> GAPATVTEQGEDITSKKDRGVLKIVKRVGNGEETPLIGDKVYVHYKGKLSNGKKEDSSHDRNEPFVFSLGKGQVIKAWDIGVATLKKGEIAHLLIKPEYAYGSAGSLPKIPSNATLFFEIELLDFKGE

Here we used the FK506-binding protein 51 (FKBP51) as a model system to evaluate whether chemically engineered proteins can be trapped in pharmacologically relevant conformations. FKBP51 has emerged as a promising drug target for chronic pain, obesity, and depression. The major challenge in FKBP51 drug development is selectivity toward its closest homologue FKBP52, as the binding pockets of both proteins are very similar, but the biological functions are opposite. Selectivity for FKBP51 can be achieved by targeting a transient conformation characterized by an outward flip of phenylalanine 67 (F67in and F67out).41−45 This conformation is rarely populated in the apo-state of FKBP51,46 but enables high selectivity vs FKBP52.47,48 To stabilize the transient binding pocket of FKBP51 (F67-out), we aimed to lock this conformation precisely by the formation of an intramolecular amide bond (sites displayed in Figure 1B).

Two positions, K58 and K60, were identified as promising anchor points for lactamization to the residue in position 67. This was expected to trap residue 67 in an out-like conformation and stabilize the β2-β3a-loop by a seven (i, i+7) or nine (i, i+9) amino acid macrocycle. Protein crystallography of the ligand-bound proteins confirmed the desired 3D structure of the synthesized and refolded proteins FKBP5116–140 F67E/K58 (i, i+9) and F67E/K60Orn (i, i+7). The protein fold, the ligand binding mode, and the conformation of the β3-strand were identical to recombinant FKBP51. Notably, the side chains of F67E/K58 and F67K60 were well resolved, which unambiguously confirmed the desired lactam bridge and its F67-out mimicking conformation. In contrast, for the lactam-bridged variants, fragments resulting from cleavage between F67E/K58, F67E/K60Orn, and F67E/K60Dab are undetectable because the covalent bond formed protects the protein from fragmentation at these sites. Lactamization within the protein was expected to shift the conformational equilibrium toward the F67-out-like conformation. This should result in a higher binding affinity of conformation-specific ligands, as the energetic penalty to adopt the F67-out-like conformation is reduced. Indeed, when we compare the Kd values of recombinant FKBP5116–140 with the synthesized and cyclized variants, we observe a 6–10-fold tighter binding for the lysine/glutamic acid cyclized variants.>MASWSHPQFEKGSMRDIVDPVFSIGISSLWDELRHMPAGGVWWFNVDRHEDAISLANQTIASQAETAHVAVISMDSDPAKIFQLDDSQGPEKIKLFSMLNHEKGLYYLTRDLQCSIDPHNYLFILVCANNAWQNIPAERLRSWLDKMNKWSRLNHCSLLVINPGNNNDKQFSLLLEEYRSLFGLASLRFQGDQHLLDIAFWCNEKGVSARQQLSVQQQNGIWTLVQSEEAEIQPRSDEKRILSNVAVLEGAPPLSEHWQLFNNNEVLFNEARTAQAATVVFSLQQNAQIEPLARSIHTLRRQRGSAMKILVRENTASLRATDERLLLACGANMVIPWNAPLSRCLTMIESVQGQKFSRYVPEDITTLLSMTQPLKLRGFQKWDVFCNAVNNMMNNPLLPAHGKGVLVALRPVPGIRVEQALTLCRPNRTGDIMTIGGNRLVLFLSFCRINDLDTALNHIFPLPTGDIFSNRMVWFEDDQISAELVQMRLLAPEQWGMPLPLTQSSKPVINAEHDGRHWRRIPEPMRLLDDAVERSS[2x];>[2x]MMTISDIIEIIVVCALIFFPLGYLARHSLRRIRDTLRLFFAKPRYVKPAGTLRRTEKARATKK;>[2x]MAVLGLQGVRGGVGTTTITAALAWSLQMLGENVLVVDACPDNLLRLSFNVDFTHRQGWARAMLDGQDWRDAGLRYTSQLDLLPFGQLSIEEQENPQHWQTRLSDICSGLQQLKASGRYQWILIDLPRDASQITHQLLSLCDHSLAIVNVDANCHIRLHQQALPDGAHILINNFRIGSQVQDDIYQLWLQSQRRLLPMLIHRDEAMAECLAAKQPVGEYRSDALAAEEILTLANWCLLNYSGLKTPVGSKS;>[2x]MGSSHHHHHHHHAAGSNNNEPDTLPDPAIGYIFQNDIVALKQAFSLPDIDYADISQREQLAAALKRWPLLAEFAQQK

Bacterial cellulosic polymers constitute a prevalent class of biofilm matrix exopolysaccharides that are synthesized by several types of bacterial cellulose secretion (Bcs) systems, which include conserved cyclic diguanylate (c-di-GMP)-dependent cellulose synthase modules together with diverse accessory subunits. In E. coli, the biogenesis of phosphoethanolamine (pEtN)-modified cellulose relies on the BcsRQABEFG macrocomplex, encompassing inner-membrane and cytosolic subunits, and an outer membrane porin, BcsC. Here we present cryo-EM structures of the E. coli Bcs macrocomplex positioning all seven BcsRQABEFG partners and multiple c-di-GMP-binding sites.

Finally, we visualize the complex’s intrinsic conformational plasticity, in which the regulatory BcsRQEF vestibule, and BcsE in particular, can resort to alternative protein interaction interfaces to maintain the activating BcsRQ partners onto the synthase’s cytosolic modules even in non-saturating dinucleotide concentrations. Interestingly, the remaining particles showed a c-di-GMP-free BcsA synthase and a more extended vestibule conformation, where the central BcsEREC* domains engage in a different dimerization interface mediated by the pairs of β1–β2 connecting loops (melted α1 relative to canonical response regulators) and the C-proximal α-helices (canonical α5). Densities for the PilZ-proximal GGDEF* domain feature markedly lower-resolution, however, the conformation for both BcsEREC*-GGDEF* tandems is still consistent with the closed BcsE state and intercalated c-di-GMP complexation. The overall BcsE fold features a more extended conformation along the NTPase*-REC* domain linkers, neither BcsE protomer contacts the cytosolic synthase modules and the X-shaped BcsF dimer is found shifted near the fifth and fourth BcsB protomer as opposed to the c-di-GMP-saturated complex shown above. Nevertheless, the BcsRQ tandem is retained as an apical complex and the synthase-proximal BcsQ and BcsR protomers engage in similarly extensive contacts with the catalytic and PilZ modules. The specific BcsE REC* domain dimerization interface and overall vestibule conformation would also be likely influenced by the lateral diffusion and BcsF partner stabilization among the synthase-distal BcsB copies of the crown. Finally, we demonstrate that through a composite, interdomain c-di-GMP binding site BcsE acts as a higher-affinity dinucleotide sensor that can adopt discrete dimerization interfaces to maintain the activating vestibule components even in the absence of direct c-di-GMP-BcsA interactions. Processive substrate addition and product release by BcsA would thus depend primarily on minute movements of its gating loop and finger helix—as observed in crystallo in saturating dinucleotide concentrations for the catalytic cycle of the R. sphaeroides BcsAB tandem—rather than be absolutely dependent on direct synthase-c-di-GMP complex formation.>[3x]MKHHHHHHSAGLEVLFQGPMVLSPYKLNLVATPLFLKPGIPYPIKVQVKDSLDQLVGGVPVTLNAQTIDVNQETSDLDPSKSVTRVDDGVASFVLNLPSGVTVLEFNVKTDAPDLPEENQAREGYRAIAYSSL;>MKHHHHHHSAGLEVLFQGPMGDVQERGHTYVTKNVTVEDGACVYLRNVIPNGETKALNNPCVLSTCYAADRKVNSTLCPNIGVDEGCHVEWTPDGVYPNCCPKHVCPSATASS[3x]

The 3 pathways all converge at the activating cleavage of C3 into C3a and C3b, and the subsequent activating cleavage of C5 into C5a and C5b. C3b and its inactivated form iC3b function as opsonins for phagocytes, while C5b initiates the terminal pathway by assembly of the pore-forming membrane attack complex (MAC, C5b-C9). To address the need for a more detailed understanding of the mechanisms of C5 activation, we have identified and characterized a family of C5 inhibitors from tick saliva, hereafter named the CirpT (complement inhibitor from Rhipicephalus pulchellus of the terminal pathway) family. Analysis of the specific binding interactions between C5 and CirpT1 suggests that the CirpT family functions by direct steric blocking of the docking of C5 onto the C5-convertase, and our data thus provide support for previous models of C5 activation, which include convertase binding through C5 domains MG4, MG5, and MG7.

To understand the interaction between CirpT1 and C5 in greater detail, a complex of CirpT1 and C5_MG4 was crystallized. The structure of the C5_MG4–CirpT1 complex was solved by molecular replacement with the isolated C5_MG4 extracted from the C5–OmCI–RacI complex. Initial phases from the partial molecular replacement solution produced a map into which a model of CirpT1 was built de novo, and the complex refined to give the model described in Fig. 4A and Table 2. CirpT1 is made up of 2 domains: A bulky N-terminal domain and a flat looped C-terminal domain. The N terminus of CirpT1 extends further, however, and engages in a 4-stranded β-sheet. A detailed analysis of the binding interface was carried out using PDB-ePISA. This revealed an extensive interface that encompasses most of the C-terminal domain of the CirpT1, with additional contributions from the N-terminal strand and 2 residues at the tip of the extended loop in the N-terminal domain (Tyr23 and Leu24). The interface is predominantly hydrophobic in nature, with His7, Tyr23, and Asn59 on CirpT1 contributing sidechain hydrogen bonds (to Asp405, Ser426, and Asn423, respectively). Overlay of the C5_MG4–CirpT1 structure onto the C5–OmCI–RaCI–CirpT1 structure revealed minor clashes between CirpT1 and the neighboring C5_MG5 domain that were resolved by a small rigid body movement of the CirpT1 into the cryo-EM density. This placement of CirpT1 in the context of intact C5 revealed additional contacts between CirpT1 and C5_MG5, including a hydrophobic cleft between C5_MG4 and C5_MG5 that Trp70 and Pro72 of CirpT1 pack into. Of note, the stretch of residues from Cys66-Glu69 in CirpT1 extend over an extension of the hydrophobic crevice between C5_MG4 and C5_MG5, but leaving a hydrophobic hole.>MFAWWGRTVYQFRYIVIGVMVALCLGGGVYGISLGNHVTQSGFYDEGSQSVAASLIGDEVYGRDRTSHVVAILTPPDDKKVTDKAWQKKVTEELDQVVKDHEDQIVGWVGWLKAPDTTDPTVSAMKTQDLRHTFISIPLQGDDDDEILKNYQVVEPELQQVNGGDIRLAGLNPLASELTGTIGEDQKRAEVAAIPLVAVVLFFVFGTVIAAALPAIIGGLAIAGALGIMRLVAEFTPVHFFAQPVVTLIGLGIAIDYGLFIVSRFREEIAEGYDTEAAVRRTVMTSGRTVVFSAVIIVASSVPLLLFPQGFLKSITYAIIASVMLAAILSITVLAAALAILGPRVDALGVTTLLKIPFLANWQFSRRIIDWFAEKTQKTKTREEVERGFWGRLVNVVMKRPIAFAAPILVVMVLLIIPLGQLSLGGISEKYLPPDNAVRQSQEQFDKLFPGFRTEPLTLVMKREDGEPITDAQIADMRAKALTVSGFTDPDNDPEKMWKERPANDSGSKDPSVRVIQNGLENRNDAAKKIDELRALQPPHGIEVFVGGTPALEQDSIHSLFDKLPLMALILIVTTTVLMFLAFGSVVLPIKAALMSALTLGSTMGILTWMFVDGHGSGLMNYTPQPLMAPMIGLIIAVIWGLSTDYEVFLVSRMVEARERGMSTAEAIRIGTATTGRLITGAALILAVVAGAFVFSDLVMMKYLAFGLLIALLLDATIIRMFLVPAVMKLLGDDCWWAPRWMKRVQEKLGL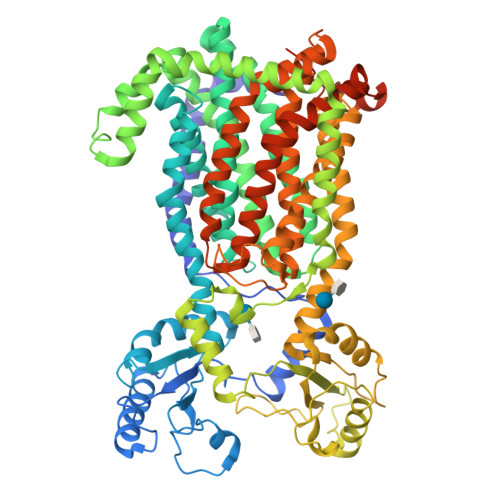GETELPDERKRPTVRESETDQRALVGVGAHHHHHH[2x]> MGSHHHHHHSQDPMAYSTREILLALCIRDSRVHGNGTLHPVLELAARETPLRLSPEDTVVLRYHVLLEEIIERNSETFTETWNRFITHTEHVDLDFNSVFLEIFHRGDPSLGRALAWMAWCMHACRTLCCNQSTPYYVVDLSVRGMLEASEGLDGWIHQQGGWSTLIEDNIPG;> PSSTMGQVGRQLAIIGDDINRRYDSE

Some viruses, such as Epstein-Barr virus (EBV), encode homologs of the mammalian pro-survival protein Bcl-2. In this study, we have confirmed that EBV BHRF1 exerts its pro-survival function by directly inhibiting a sub-set of pro-apoptotic Bcl-2 family proteins Bid, Bim, Puma and Bak, presumably ones most critical for the virus. We have therefore determined crystal structures of BHRF1 in complex with its key targets, the BH3 domains of Bim and Bak. Our three-dimensional structures show that these interactions closely resemble those seen with mammalian pro-survival proteins such as Bcl-xL.

Recombinant BHRF1 bound a 26-mer Bak BH3 peptide (KD = 150 nM), but only weakly (>1 µM) to Bax BH3. Consistent with the binding data, we observed that BHRF1 could directly counter Bak, but not Bax, when these proteins were expressed in yeast. Taken together with the previous reports that BHRF1 interacts with the full-length Bak, but not with Bax, we conclude that BHRF1 can keep Bak inactive by direct binding, but must inhibit Bax indirectly, presumably by its ability to sequester BH3-only proteins such as Bim. Bak BH3 binds in an equivalent manner, and the two complexes superimpose with an RMSD of only 0.6 Å over the entire BHRF1 backbone indicating their similarities. As the characteristic hydrophobic surface groove was absent in unliganded BHRF1 due to the close proximity of helices α3 and α4, significant structural changes are required in order to accommodate Bim or Bak BH3 domains. These changes affect mainly α4, which is at a 120° angle to α3 in the BH3-bound form, compared to the near anti-parallel alignment in the free form. The side-chain interactions contributing to the BHRF1-BH3 complexes are equivalent to those observed for mammalian pro-survival proteins such as Bcl-xL, with the four conserved hydrophobic BH3 residues of Bim (I58, L62, I65 and F69; numbering based on human BimL) protruding into pockets within the BHRF1 hydrophobic binding groove. Similarly, Bak residues V74, L78, I81 and I85 (numbering based on human Bak) interact with the BHRF1 binding groove. In addition to the hydrophobic interactions, BHRF1 R100 forms a salt bridge with Bim D67 or with Bak D83. The conservation of aspartic acid in the mammalian BH3 ligands suggests that this interaction is of particular importance for complex formation, and indeed a BHRF1 R100A mutation reduces Bim binding and abolishes interaction with Bak.CutA1 is universally distributed in bacteria, plants and animals. CutA1 from Escherichia coli (Ec-CutA1) is related to the copper-tolerance mechanism. CutA1 from Homo sapiens (Hs-CutA1) appears to be necessary for the localization of acetylcholinesterase at the cell surface. The functions of CutA1, however, have not been well clarified. It is known that CutA1s from Pyrococcus horikoshii, Thermus thermophilus and Oryza sativa unfold at temperatures remarkably higher than the growth temperatures of the host organisms.

In this work the crystal structure of CutA1 from the psychrotrophic bacterium Shewanella sp. SIB1 (SIB1–CutA1) in a trimeric form was determined at 2.7 Å resolution. This is the first crystal structure of a psychrotrophic CutA1. The overall structure of SIB1–CutA1 is similar to those of CutA1 from Homo sapiens, Escherichia coli, Pyrococcus horikoshii, Thermus thermophilus, Termotoga maritima, Oryza sativa and Rattus norvergicus. The root-mean-square deviations (r.m.s.d.) of the Cα atoms for Ec-CutA1 and Ph-CutA1 against SIB1–CutA1 are 1.00 and 1.08 Å as a monomer, and 1.11 and 1.17 Å as a trimer. In the case of SIB1–CutA1 from a psychrotrophic bacterium, Gln residue (Gln39) is inserted into the β2 strand and the β2 strand is divided into two short β strands. Another peculiarity is that the β3 strand of SIB1–CutA1 is kinked by Pro residue (Pro58). The intertwined interactions among β strands of SIB1–CutA1 seem to stabilize the trimeric structure as in other CutA1 proteins. Furthermore, we found that the subunits in the trimer are firmly locked to each other with the highly conserved aromatic residues, such as Tyr45, Trp47, Tyr81, Tyr98 and Trp101, in SIB1–CutA1. Therefore, we propose that CutA1 is stabilized by the aromatic cluster in addition to the β strands and hydrophobic interactions. A thermal denaturation experiment revealed that SIB1–CutA1 does not unfold completely at 363 K at pH 7.0, although Shewanella sp. SIB1 cannot grow at temperatures exceeding 303 K. These results indicate that the trimeric structural motif of CutA1 is the critical factor in its unusually high stability and suggest that CutA1 needs to maintain its high stability in order to function, even in psychrotrophs.

>MYKPEQLLIFTTCPDADIACRIATALVEAKLAACVQIGQAVESIYQWDNNICQSHEVPMQIKCMTTDYPAIEQLVITMHPYEVPEFIATPIIGGFGPYLQWIKDNSPS[6x]NAPHTHALENE | C10 H8 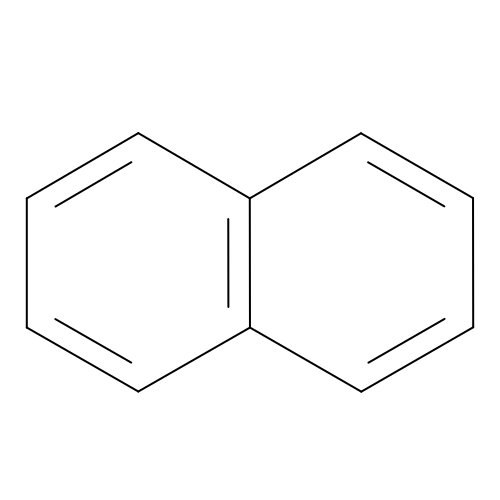| UFWIBTONFRDIAS-UHFFFAOYSA-N>[9x]MIITQVELYKSPVKLKEPFKISLGI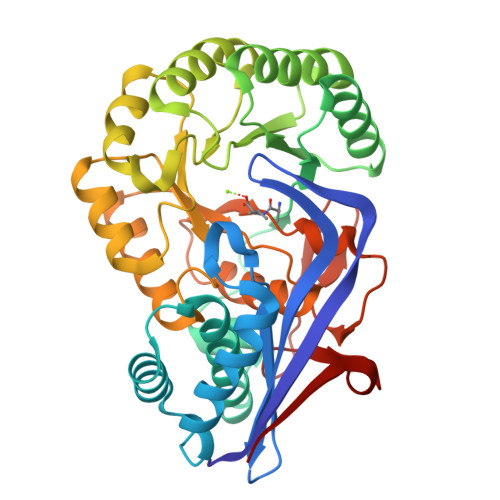LTHANNVIVRIHTASGHIGYGECSPFMTIHGESMDTAFIVGQYLAKGLIGTSCLDIVSNSLLMDAIIYGNSCIKSAFNIALYDLAAQHAGLPLYAFLGGKKDKIIQTDYTVSIDEPHKMAADAVQIKKNGFEIIKVKVGGSKELDVERIRMIREAAGDSITLRIDANQGWSVETAIETLTLLEPYNIQHCEEPVSRNLYTALPKIRQACRIPIMADESCCNSFDAERLIQIQACDSFNLKLSKSAGITNALNIIRLAEQAHMPVQVGGFLESRLGFTAAAHVALVSKTICYYDFDTPLMFEADPVRGGIVYQQRGIIEVPETAGLGAGYQKDYLSGLEKICIN In eukaryotes, the ubiquitin‐related modifier 1 (Urm1) pathway is responsible for the synthesis of 2‐thiolated wobble uridine (U34). Uba4 is a two‐domain protein containing an adenylation domain (AD) and a rhodanese‐like domain (RHD), which are both essential for the dual function of Uba4 in sulfur transfer and ubiquitin‐like conjugation (Furukawa et al, 2000; Huang et al, 2008; Schmitz et al, 2008; Leidel et al, 2009; Noma et al, 2009). Uba4 activates the C‐terminus of Urm1 via an ATP‐dependent adenylation step, receives mobilized sulfur from the Nfs1/Tum1‐relay system by its RHD, and subsequently forms thiocarboxylated Urm1 (Urm1‐COSH; Leidel et al, 2009; Noma et al, 2009). We heterologously expressed and purified Uba4 from Chaetomium thermophilum (CtUba4), a thermophilic fungus harboring highly stable proteins, well‐suited for X‐ray crystallography and other in vitro approaches (Bock et al, 2014).

Therefore, we generated a Uba4C202K mutation to convert the labile thioester intermediate into a non‐hydrolysable iso‐peptide bond between the activated C‐terminus of Urm1 and the ε‐amino group of the introduced lysine. Indeed, we found that Uba4C202K forms a covalent bond with Urm1 in the presence of ATP, while other Uba4 mutants (C202S, C397S, 306GGS314) led to the formation of non‐covalent Uba4–Urm1 complexes similar to wild‐type Uba4. The covalently linked Uba4C202K–Urm1 complex formed well‐diffracting crystals resulting in a structure at 3.15 Å resolution, and its atomic model was refined to R/Rfree values of 21.1%/26.2%. The structure revealed two Urm1 molecules with slightly higher B‐factors bound to a dimer of the Uba4 AD (Figs 3B and EV3A), while no specific density could be attributed to the RHD, which although present in our crystals, appears to be mobile at this specific reaction step. In contrast to Uba4 alone, the Uba4–Urm1 dimer is fully symmetric and the AD interface falls on a twofold crystallographic axis. Interestingly, the C‐terminal GG‐motif of Urm1 is positioned in the same groove that was occupied by the linker region in the unbound Uba4 structure (Figs 3D and EV3B). Importantly, a helical region localized adjacent to the ATP‐binding site (aa 72–88) in the structure of apo Uba4 becomes disordered and flexible in the structure of the Uba4–Urm1 complex (Fig EV4). In contrast, the loop containing Cys202, known as “crossover loop” in other E1 enzymes, becomes structured in the Uba4–Urm1 complex and an electron density can be clearly assigned to the covalent peptide bond between the introduced Lys202 and the C‐terminal glycine (Gly111) of Urm1 (Fig EV3B). Therefore, the Uba4C202K‐Urm1 structure represents a unique previously uncharacterized reaction step, mimicking the thioester formation after the release of AMP that can serve as a model for this reaction intermediate in all other E1‐UBL and SCP systems.

> TQKSLSKEEIERYSRQMIVPGMGKEGQLRLMNAKVLIIGAGGLGCPAAQYLAGAGVGTIGIVDGDSVETSNLHRQVAHATKRVGMLKVDSLITHLIEINPLPVYVPYRFDLTPQNAAQIIKPWDVILDCTDNPATRYLISDVCVLLGKPLVSAASVQKSGQLIVLNCPPTPQGVVNKKAAPCYRCCFKKPPPPSAQTSKGEAGIMGPVVGMMGVAQAGEAIKILVSQLHMPPKEGEEVSPEKNLVQPTLLIYTYDLNSAIGPYSFRALKMGGRKKDCFACGENSTLTLDGIKSGNPNYVQQ;> IPITVDFSGGLEMLFDNQRRHSISLPAKDTEGKPVTIAFLIDYICKKLMKDPRTDLFVLDNHIRPGILVLINDADWELEGEEAYEIQPNDNILFVSTLHGG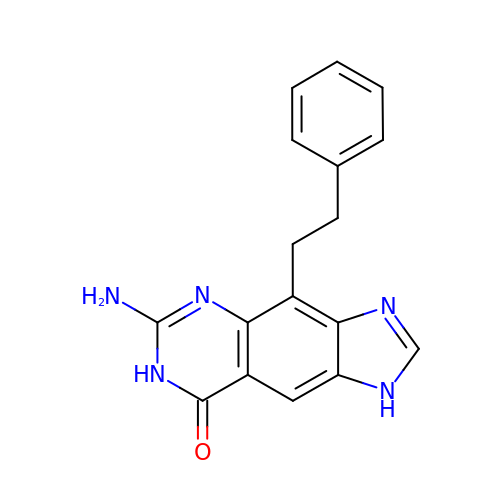6-AMINO-4-(2-PHENYLETHYL)-1,7-DIHYDRO-8H-IMIDAZO[4,5-G]QUINAZOLIN-8-ONE | C17 H15 N5 O | PBZAIUVFRISTSZ-UHFFFAOYSA-N> KYSKRIAWMKTTICDSLQLKDMIVEESFQYEKNKNLLEQFLSGEGLNKIFAYYQVQEQAQNDDIKDTGAQDPVLFFTTGDLEKIQDKAVWFLRITNPADDKKKASQQDGNDNDIIFGEITPNTVPMLNALMESVYSRQIDHIITEKIQFWGVAEEEQVLEFQQHSNKFSSEVREAINLMSPGTEHFKLDYEAISGLSESEKMQHYEMKFNEWINLISSQLNDDSEVRKDEKDAGPATELIYWRSRMQKITNWSEQLKSKDFQIVKASLQRHKNHDNQRPRGDESLSKLMMEYNRLDLLLTDKLNEAKDNVKYLTTLEKFIEPLYNGTPQQIIDTLPALMNAIKMIHTIARFYNTTDKMTGLFIKITNQMIKNCKDRILNKKDNGDNPSLYKMIWEQDPAELIEVLGSCIKLYCEYKKCYNDTKEKVADMPKGKTFDFSDAQIFGKFDTFVRRLQKLIEIFSNIQQFNALAKHNLEGMDVLTNKFKKIIDDFKKKGHNLLDTANNKFDRDWVEFNVEISHLDGELQNFIDNNFNRFRNIEYSLKLLHKFQSTIKRDSLKHNLTSRYNAILHNYATELDTIQRVFQDQKSNPPLVRNMPPEAGKIIWARHLFQKITGPINIFPENVINSTEIRRYYGSYNTLGKQLTIYEMWFYQDWVNKIEQSKAALQATLIVRHDENKKLYVNFDLEIMQLIREAKCLDRQGIEIPESARIILLQEDKFKTYYNELLYALKEYERINSKIKPICKNLLLPHIEDLDLKLRPGMVTLTWTSMNIESYLYYVHQGLKKLEQLIINVNDIIENRIENNLKTVSKVVLVHLPQDTKPLSLDSFVQLQEEYINSKTDFLTSKNVEVERAVDDLLQTIMLYPLDPHVDPVLPEETKRIKRYYFWYFYQALLNSTQNSLNAMKYRVCGKKIPGANTLQNLKPFFQVEVQLNGDKVTLNPSLQEIQKSINRAATAVLRCSKHLYNWDQQNKDSTDKATFYDMIACDKEIVKVILLLTGSIQGTKNKVNEFLSGFTKFEWLCKESIQESIKKFSKNGPTLQNYEDQLKKFSQIEEEIEKIVPTYKIGAMELMTHNICTSLSTWAKEWKLQYSQDLHKRARQLLDSLTEQTKMLSTKLSKPVKDIDSLGYVMETLEQIRKEQAEIDMKFNPVQEMYSLLDNYLPGGITDKDEMDARSLLRRNWDILIQQAEIKGKEYQHKQAIYLKELKQSIKDFTNQVSIFRRDYEKNGPMVEGISPAEAMERLRRFEDEYDVKYQMYKINARGENLFGLQNQKYPELEKTDAEIKNLNKLYNLYDSVIKNIQQFKEKSWQDVSKDDLAKMEEDAGKYGEQCSRLPKDLKEWQAYRDLKNYIDSLREQLPLIISLKKPSIMPRHWEKIKEITNTKLNYENPDQFYIEEIMGAKLLDFREDIEDITESADKQLKIRTGLDEINLYWNDMQFQFGIWGKRDVPCMLNGLIVGTILERLEEDQLQLSTFNSQRHVTPFKAEVENLIRTFSDVNDTLDMWVKVQKLWTSLEPVFTGGDIARQMPLQAKQFQGIDKNWMKIMEKAVETKKVIPCCQNDMLKDFLPDLNRKLEDCQKMLEAYLEGKRKKFPRFYFVSNPTLLKILSQGSEPTSIQEDFEKLFDAITKVTFESAKDKKNPALKQITQIQQVIGRNEENISLTGYYVKCEGNIEDWLKKLEQNMQQTLKDIASAAAQQVFQVGLKEFVSSQASQIALLGLQILWTSKVNEGLERLSRNERNAMDIKRNEIKEHMNILSSMCLEDLNGAVERTKVETLVTIQVHQKDISMDLKCKDVNDFEWQKQTRIAWKTDIDECIISITDWDSPYSYEFLGAKERLCITPLTDRCYITLAQAMSMYYGGAPAGPAGTGKTETVKDLGRTLGVFVVVTNCSDQHRYRDMAKIFKGLVQSGLWGCFDEFNRIDLEVLSVVAMQVESITTARKQHMKKFMFPEEEIEIELIPTVSYFITMNPGYAGRQELPENLKVLFRGVSMMVPDREIIIKVKLASVGYLQIDLLAKKFNVLYRLCEEQLSKQRHYDFGLRNILSVLRTAGNTKRQEIKSDEEMLLMRSLRDMNLSKLVADDIPLFNGLLADIFPKLKEVPKKLYPDVEKKIPEEINAESYLINTPSFQLKIIQLYETCLVRHGFMLVGPTGSGKSTIMKILTEVLTKLGSPHKIVIMNPKAITAEQMYGVKSEISDDWIPGVFSTIWAKSNNRALKHTTWITCDGPVDAIWIENLNTVLDDNKILTLANGERIAMTENCKVVFEVENLNNASPATVSRCGQVYVSPTDLGYEAVIEGWIRNRKASGRAEESDKLGNILRKYLINMRFIELQSKECKEPMMDTSPVISVINILNLLTGCLQYFVQTQRTLSEQEYEKFIVYSMAWAIGGIYEAQDRVRFHELLLAKNAPIPQKGKENETVFDYYVSQDYLDWKICSPEEWVPPQSLQFSQLLLPTLDSFRAEMLLNFILTQPKSHTCSNSALLIGGSGTAKTSSVLLYCNKFDPQKMLFKRTNFSSATSPFMFQSTIEAECDFKVGKEFAPPGNKMMTIFIDDMSMPFVNKWGDQITLELVRQLIETGGFYMLDKTQRGNQRKMKNLQYIGAMNHPGGGRNDIPNRLKRQFFIFNMILPLSIEGIYGPIIKHMFKQKYFSDSTYKVIESLTSATIALWNKVKSTMLPTPAKFHYVFNMRELSRIFKGILTCKKDTINDAPKSMKIKPELFLVGLWRHEAERVLADKLVNNKDKDTVMGYIQEVSLESFSQIENEILEKYSSEKTFLFCDFLRPDVINEDGIIEEEAPKIYEAIDSLTELRKRCNFLLSFYNDRNPSKKMPLVLFDDALKHLLRISRIIRQPRSSGLLVGVGGSGKQSLTRLAGFIGKNLIQQIIVTKTYSDKDLKEDIKKGFDDAGHLGKQVTFLMTDSEVKKEEFLEYINMVLSTGEIPNLLAKDEREVWLGDISQ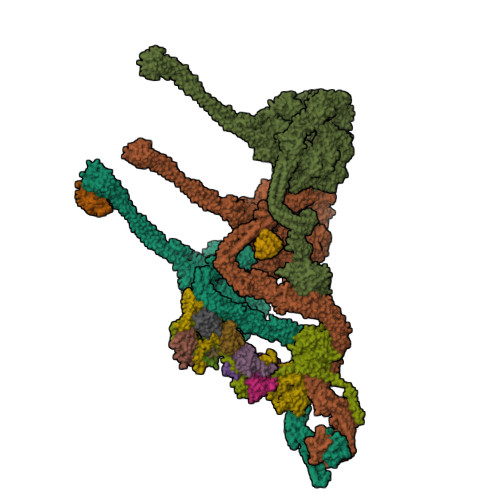AYCKEKNLGNIDPPQSELWTYFVDRVRDNFHIMLCFSPVGQKFRERARKFPALFNECTIDWFLPWPEEALVSVAETFIKNFDKLDTKEETKQELMKHMGNVHLMVNEICDEYYQKMRRQVYVTPKSFLSYLNSYKTLYIEKYDELDQQEESFKIGLNKIQEATITINQMEISLKEEEIQLNEATEKTNQLLANLDKESKKANQKGEEVAATNKQCEIQAEQISKEKEEAERELEAALPALRRAQEAVDSIESKDIVELKANKKPLDIIKYIMDAVLVFFKARLIPIQIEERVFNKKEGKAVLFLKESYDESGIQTLGDMNFMKKLKEFEKDSINEETIELLEPYLNQSEDWFNDTFATKASKAAAGILKWAFAIYEYHQKSKIVKPKRIQVAIAEGRQAIALKELEKAREDLAQIQAYIKNLKDVYTKQMEEKNELEMKAAKTKKKINTARTLITSLSGEKDRWGKGAQDISDQKRKLVGNVSLSTAFISYCGPFNAEYRNKLAQQRFVVDMKKRGVPVTPGLELTSFLIDDATIGEWNLQGLPKDDLSIQNGIMVTNSARYPLFIDPQGQGQNWIRNKLSASIIPERCITTLSHPKFKDMFLKYCMESGLTLIVENIENEVDPMMDPVLERQIIVKGKTQFVNVAGTEMELSKEFKLFMTCRLANPSFSPELSAKTTIIDFTVTQSGLEQQLLGKVISKEQKALEDSLNQLLADVNQNQKDLQRLDKNLLERLINSQGNLLDDTELMDVLNNTKTQAKEVAAKLIDAEIKTKEINEKREQYRPVAIRGSAIYFTMIEVSLVNWMYNSSLEQFLKLFIESIDLSEKAQLPSNRVKNIISFLTFHVYRYVNRGLFEKDKITFILMMAFKILTTAGTISSGDVSLFLKSGDALDIKSERQKQISYLEDNQWLNILALSKHTFSGQTLPFFKELPDLISRSENQWRNWIDKNDPENFPIPDFAESINQEKEIGSFISLCLVRSLRNDRTLIATQNFISNVLGKEFTDPISYPIEGIWQESSNMDPVLFLLSAGADPTSSIDELAKKKKKFPCEKVSMGEGQERVARQVIMKGFVEGGWVILQNCHLGLKFMEEIETLVSPINQIHEDFRLWITCEQHPKFPLGLLQKTLKVTNEPPKGLKAGLYKTFTTIITQEFIDKVDHSNWRSLIFTICFLHSIVIERKKFGPLGWCVPYEYNYSDLEASLLYIEKYLTNLMSTPQPNSHNLPISMNVVRYMICEVQYGGRITDDLDRELFITYGETYLKDGIFGNDYFFYDIMVDGSGQKFKYRIPQNPSAELIKYQEYIAKVPTVDNPEVFGLHSNADLTFRLKESKEMINTVMETRPKDSSVGGGKTREEIVQDKAKDMLKNLPPDYNDVEVRELVSKLGGPNPKTSTERGMTVPLNIFLYQEVTRMQRVIGLVRKTLQDTILAIDGQIIMTPEILEAINAIYDAKVPNSWLYDPSGAEISWLLPNLGSWSTSLSDRNKQLNDWLRSGQRPILFWLTGFFNPQGFLTGMKQEVTRNHKKGDGKGGEAWSLDDVVYSTTVKEREKEKDIEQPPAEGVYIKGLYLEGCKWSKNGLDDSDPKKIFADLPILHVSAINKKKTNEQDRMSNTYLCPVYKYPKRTDKYLIFRVGLPCEGSNNPSHWKLRGVALLCST;> MGDHSQKDSPEDFIINRLSQALGIQKEKIKKSLETQQDDKGEVTNKDEFQGFIQQDNSTNILWVSGQSEKCTFYYGQLPPIDKFKKKGIAVIKLGLHKLTNENVAKDVVVVEITNNLLEHLNSVFNEIMSPVMQNPLNQQGWTDLVAKDLMEKFNNYVAQVYVLLGQIKGKTMLPLPSHKLTSSDTTPDKDKAHVFEGSIITWTKQIKNVLKLEPEQLLKYGNDPGPLAEIEFWQNKRDNLNLIDSQLKSVEVQNILHFLDNNKSTYTTPFTKLQAEVKKARLEANENYRYLFTLKDLFSKLQESQPSDFPTLYELFIPIMHTILLIYNKSKTYNQPPRLVVLIREICNAIISNAQAFVDKDTIFSLIDSKETTEACDKLQVTLDVCSKFKDAYFEYKAKAGGNWKLTSNALFVRLDSFLERCQDILHLTNTIVQFNKLEKIELGGTKGKTLTESIAQIFKEFEEAVQAFTSVSYDIMNIAEKKFDDDFYEFRSKIKELERRLASVITQGFDDYDTIYGRFKLLDNFEGLLTRPIIADELEKKHIVLLEMYKQDLKQVQSIFLEGKQFVDSMHENAPLFLNMPPIAGALTWCKSLRDRIQEPIEKLAQLGQGITEREEYKDVQKLYTSITKSIKDYEDQKILSWEKEVEDSSQDKLKQTLLCKDENDLIKVNFDPSLVRLLKEVKYFLLLRLEVPTTAKDIYTKAETYRTQIVALDMIVDNYNHIKTCLLPVEEPLVKKKIQDMEEEVKPGIEEIRWKSTNIDQFISKSKSIVDQLFETVNKMKDSLQKIHKSLANFNVKIIERKNRPMSPDDYDQFLKAIFSNKLTIVKDNGNQIQKLVKEVLDAVKADKKQNSWKNYNDYVNVIVIEGISTAIQTALLHLNEQINPVFIKRNDISPLFDIRLELGQSGIQFDPEIGESSNQLTVRNTIRNWINDFFNIAGTIQRLDTTMPGDFLQEIRSFFEIKQCLAMITQNLEWIENECNQFRARFDTYSYLWTEDEQISFNRFLDENEPKDEDGKGGDDDEGENTEKQNPLLKGCRAKIPNLDLFDEKITHLKAIQQEISRIKTPEDISWLRINLQPMKTALDARVTRWIRVYTDFLVNQFRTTQKNLLDFIEKTKDGIKKNPADHENLHDKKLLMSVMKVISDVKDVEPRREGIITRMKEMVTKLKKHNVPITEKGTDDPLQQIDNANSNFIEIYGRVFKVKADIIPLQAEETQNIKRDLDIFMKEVESFRKEFMQKLPFDYTESMGYENINNAYDTIMVYYHKLTAIEGRALEYNNLEKLFELQKSNYKQLKDCMNDLKNLKTMWDAIALIHFQYNDWKTKPWRQIKADILLDTNKTLGTQIKNLPKEIRNFKGYNVIVEKVKNMGTVLPLVSALHSEFMEDRHWSQLKQITGTVFDHNSLSFYFEDILALNLYKYENTVNEIVDVAQKEAKIEKKLKNIEQWWSKQVFEFTEYKETKTFASLDNMMEVLDQHSLDLMGMKSQGKYVEFFYDRVEDWREKLGRVDVVVNEWLKVQKNWKILYNIFLLSEDIRMQLPEDTKVFEGVDKEFKDMMSEVSANPSVVEACTIERRDVLVGWSQAIKKCEKALNDYLEQKKKSFPRFYFLSNQSLLTILSNGQNAPKVCEYLGDCFDGLKTLTFEPPANPAETSKVGIGMISKDDEKVPFSSKFICEGAVEHWLLNLEFRMRETLQEILEGAKNTADLWDSGDKPREEWVEGYNAQIALLTTTIVWTEDVGRAFEDLAGGSETAMKECQKLIEVRLENLIKKVRGDLHILERWKIINIITIDVHSRDVVEKFVIQKVSEAESFAWLSQLKFYWENKPDSDMHLRQTLRFPWEKDKNKNKCIIRIVDWFRFYSYEYIGNAIRLVITPLTDRCYITLTQALNLTMGGAPAGPAGTGKTETTKDLGRAIGIPVMVFNCSDQMNKDSMAQIFMGLSQSGAWGCFDEFNRISIEVLSVVSTQVKCVLDALKEKKTKFSFVEEGEIQLQDTVGFFITMNPGYAGRTELPENLKALFRSCAMVVPDLALICENMLMSEGFTMARVLSRKFVSLYMLSRELLSKQKHYDWGLRAVKSVLRQAGKLKRGDPDMPEDPLLMRALRDFNMPKIVTDDKVIFRRLIGDLFPKLDPPTKQNPELKKIVQDTTKKDMGLVAEELFVTKVVQLAEILEVRHCCFVIGPPGSGKTCVWKTLIKSYINSGEDAEYDTLNPKAVTSDELFGAYTKTKEWKNGVIAVIMKNQVKNEEKYKATHMHKWSVLDGDIDPEWIESLNTVMDDNKVLTLVSNDRIFLTPQMRLIFEISNLRNATPATVSRAGVLFINETDIGWMPYMNSWLERSQINILKQQKEMANMPEYPVIDDVAKSVFYRCFQSYFEQNIDVHDKNRVRHICPMVDIAMIQTICTILDALLIQHLPKLKQMKEEDEKQALEAFFIFAGLWAIGGPVGGGQDDSKDMKEFNTVWKGAAKVKFPEQGLCYDYYYDINENKWNTWKVEDYLPNDQPLFSKIYVATIHTTRLRYMIDIHLQRRKPILFIGSAGTGKTAVVRDYLNSTRPEQVSHKTINFSSFTDSLALQKNIESMVEKKNGRNYGSATNKVLICFIDDFNMPYVDKYGTQSPIQLLRLILDYGSIFNREQLEERKFLQDLLFFGCLNQKSGSFTVDLRLQRNFSVFSMYTPSSDVIKTIFGSILNAHLSTIDDKAQKMAFKLVEATYFTFDKILKNTTAFAPSAKRFHYQFNFRELARVCEGICRTTPGQYSGGDQGKLVRLWAHEMKRTFEDRFIANEHVEFFRRYLTEAISKCIGEFPETENPIAEPLIFTGFVAAHQGLDQQYTQCTIPVLKRVLDDKLEEYNEVKAQMNLVLFQQAMEHVSRICRILDMPGNNALLVGVGGSGKQSLCRLSTFINGFEIDQLVVTASFTINDLRNNLQEIYKKIAKPNSIARVFMITDSQIKEEQFLIPINDMLNSGWIFDLFPKEDMDSLVSGVRNEAKGEGVDVNNLTALTSYFLDKIRKNLKVVLCFSPVGDTMRIRSRKFPGIINNTSIDWFHPWPHEALIDVAFRFLEEIEFPTEEIRQSISLNMAKVHSSIDTANEKFLKLERRYNYTTPKSFLELIDFYKKLLTEKRETIQRQIQRYEMGLNILAETQNKVQGLQEELKVKMVEVNKQREETDILIEKVGKESALAEEEQTIANAEEEKTNVAAAEAEKISKEATEALAEALPALRSAEAAVDCLKKPHVTEMKNLGSPPAGVIVTARVVLILFNQGITLNDPDEKVWKKAVTFMNNPQAFIDKVKSFDGENIEPNIIEQSNKIIQDPSKKFNEKDMAGQSYAASKLCAWAVNIVTFNKIFKQVKPLQDAQKQANEILEEKKKELAIVKQRVAELNARVNSLKRQLEEAEARKMIVEQDAARCQSRLSAAENLVNGLAGENKRWTQNVKFLKENIKSMIGDSLLASAFVSYIGAFSAKLRLELWKNTWLPDIIEKGIPITEGIEPLKILTTEAIKSKWKNEGLPADPMSLENAAIITACARWPLIIDPQLQGSTWIRGKQGENLTTISLSQPKWLGALTSSISSGRAVLIEGIQQEIDATLDPLLQRAVKKNGNQLQLEIGGDPIDYDPNFKLFLMTKLINPHFRPEIAAQCTIINFIVTESGLEEQFIAMVVNIEKNELEMAKQDLVKKQNEYAVTLDKLESDLLQSLSEADPATILDNTELIQNLDKTKKTTIEITEQQQKAKVTEAEINIQREHYRVVAAEGSMLYFLVISLSVMDHMYQYSLESFITFFFKAINRTTVRDENRIPTLILNIRQTIYQWISRGLFEKHKLIFLTLIVFRLMQKKIIDVAYEVAEMDFLIKCPARPGVENTLDWLPNISWDQIQGLINLEEFRNFAHQLEKEAPNRFKDWYNELQPEDQKLPLDWKRLDSMPFKKLLVLRCLRPDRMTISLNNFIRAVLPQGDAFVEMDQKLAFSEILESVINEDSESTIPIFFILSPGSDPVKEVEKIAKKKRIEPGKNFFNIALGQGQDEIARRRIEEGNKEGHWVMLQNIHLMPTWLIELEKILDSYSGEAGGGNSEFRLFLSAEPSTGIPIGILDRSIKLTNEPPAGLKANMKRAWTYFSKEEIEDKDPKIKSILFALCFFHSTLIERRRFGPKGWNMSYPFNMGDLRDSYLVMNRYMEQNQGGKVPFNDLIYIFGEIMYGGHIVDDWDRRLCNSYLFNTMHEQLFDELELFPYIEGKGLSFKVPGQNPYEKYIEHIETSLKQETPLAYGLHPNAEIGFRTDQCKTLFNTLLELMPKEQSRDEKSSDIKSSNEMASDLIKQLLEDSELKNKIFNMEEIKNKIDAENKGPYQNVFLQEIEYMNALLSEIVKDLEEIGQGLSGLLTVSENMEMIIESIALSRVPASWQKLAYPSKRGLQSWLANLFQRIEQLNIFRDDPYSIPRVVMISRFFNPQSFLTAIMQVISRAKAYELNKLYIQTEITKRSIEEIEGAAKEGAYVYGFILEGARWDYQLGQLEESKPKEMFSVLPVTYCKAIPLPPEGKEDKSLYQCPVYKTEDRGNTYVFTAQLKTRFPPRKWILAGVAIIMDVEGVSD;> PLVWTQLKQTGTTQPTARSGHTIITVGKTHIMFGGLDNDKNNYKDGKIAPNNQVFTLKLTQNNCEWRQIACQGDVPLPRCYHASCAISADKMLVFGGSYTSNLRFNDTYILKTTSYQWSKPANQISGGEPKNAESKIGAPQPRYGHSATFFEGKVYIFGGHGGINYQRLAFNDLYVLETENFEWTRLEPKGNPPDPRGGHSAAMMANKPQLMIFGGWSFTSQYSNIMIYDIEKDEWVDPEIAHEIPKWNLSGIMAPSIPSWKYFIFGGSVGSFEEGGNRTNSRFVDDSFVLDIDTLSWSSINLEADETSKAVCKPRPRESASIFYDSGESRAIVFGGWANNWLNDLWALNVSTITGPIFSIKPALGPLTGKTKVLIEGDGFKDTQNISVKFSGGKLEKEVNGTFVNEKEISCETPTFDYPRSVEVTVCMNKGDYTITKSAFTYTKADKTIAYGPGLLTENLIGVQTTIVIQARNGSDEFVVTIRNPAKIKKEEEVKEGDKANTKNTIKEDEEEEGEDEEENKKKKEAEKNDLTGSAVMNYISKQLKDIQEFIENTKENIEIRNKNISELINVMINLEKVRVKNDDDVLTLDTVEEMLNFLKKKKDSDIKKCKKLQEEWKNLAKMAQAVKKDIQNPVKTESDKTKENIKKFEEITLKEYANSLKKESFYKTGVSESFKRIGEVKQKVDEFEVQLNQYEDFARIGSKKLMEQIRTDVSSVEKLWVRIEISEKTMDEYKKMKWGSINSMDMEDEIKKLRKALTDLRGIDKRSNAFIGITEELKKWATFLPLLGELKDPSMNSEDGRHWKKLKDLVKKEFDVSQELMLEIIWDLKLFDYKDGIEEITDQAKQELKMEKALKKIIDFWRDIEFELVQHKNTDIHTLKMSEENFETLEDHQLQINNMLLSKYVAYFEKEVEKWKYDLGSVYDVVQLLLEVQKTWSFLENLFEVKRELPNESAQFVGIDKDMKEIMQKGCDIKNCLKFCTIEGMLKRLENIQAQLKVCEKALNEFLDSKRRAFPRFYFVSVNDLLDILSNGNSPAKINRHMSKIFQAIDNLQLKEDSSGGRPTLKMISCVGTEEVDFSSPRLLQGKVESYLKDVIDTMIGTLKSVANSSFKNFQSMTRKEWLKSDPSQITLLVNNIIWSKAVEDCFLKLQSGDINAMKLFLDESIKQLTELIGMVQGDLSKPLRQKIMCLITIDTHSRDVVHRLINEHVRKAEEFQWQSQLKFYWVDNDAKIKIADARFVYNYEYLGNGPRLVITPLTDRIYVTATQALHLKMGCAPAGPAGTGKTETTKDLANALAKACYVFNCSSEMNYESMGNIYKGLASSGCWGCFDEFNRLLPEVLSVCSVQFKAVTDAIKQNVERFIIEGDEISLDPTCGVFITMNPGYLGRAELPEGLKALFRPITVVVPDLELICENMLMAEGFIEAKILAKKFVTLYMLCRDLLSKQLHYDWGLRAIKSVLVVAGGFKRSEPEIAEQALLMRALRDFNIPKIAFQDLYVFHGLLGDLFPGINIKPKKDLDFEKIITDVCIENKLDPDPEFVLKVVQLSELLAIRHCVFVMGPPGAGKSTTWKILAKAQDKTNKKTTLIDIDPKVVSTKDFYGYNLPSKEWKDGLFSKMLRSLAEQPDTNPKWICLDGDLDANWIESMNSVMDDNKILTLANNERIPLKPHMRALFEIRDLRFATPATVSRAGILYISDEVGYQWRSYVKSWIKQEFSQDQEMSKNLDTLFGKYVPDTLDHIKKHCRFLVPVSPISQVISICKSLQTLLKGDVKNLEYLFVYALIWAIGGALAEKDSIDYRKDFSTWWKGAWKTAVKFPSKGTIFDYYVDQSGDSSKFVEWSKRLENKEFDPQVETMGNITVNTIETLATTEFIKSYLMVKHPSLLIGNSGCGKTQLAKGILKEIVQAKPENYAYQLINFNYYTDSTYLQGQIEQTLEKKAGRQYGPPGKVQLIYFIDDLNMPQLDAYDTQTAIALLRQLADYGHFYDVSKLALKDIINTQVLAAMNPSAGSFFVNPRYQRHFWTISIPFPDNESLSLIYITFLNGHLKRFKSTIQEYSNIIVRASLMLHQAVTQNFRKTAINFHYEFNLRHMSNVFQGLLLSDPNKFTEPDKLIKLWIHECERTYGDRLVSTDNLKTYKENIFDIVKKSFSKFNFSRYFGNNPENLIYCNFIAGINSDRFYDQMPNNEMEKHISEALKEYNDNNAFMGLVLFEDAMKHVCRICRIVLPSSGHALLVGVGGSGKQSLSKLASFIMGYTTFSITISATYSMVDLRNDLQQLYFKCGPKEEGILFLFTEGQITNERFLVYINDLLSSGEIAELYTLDEKEAMINQVRAKVKGEGKPDTRENCWNWFIDQVKKNLHMAICFSPVGDMRRRARQFPALVNCTVIDWFQPWPYEALFNVAKSFLEPVDLGDDKVREAVVKFMPFSFTLVNDLGLKLLEQERRYAYTTPKSFLELISLFTNMLAQKRESLERNKERYETGLVKLKETAEQVAIIEVEVKEKQVEAEAKKKEADAFAEVVGREKDKVEKENSKATIEADKCGLIKQNVEAQKSSTQQDLDAAQPLVEQAKSALNSISKKDFQQAKSFASPPAGVPEVFAATIYLLAGYFNEAIEIDKNKKPKDVSWKSSLKLMKSPEEFMEKLLNFKDVVDANQVANVNIVKNQYLNMPSFTPEQMASKSAAAKGICSWVVNIVKYYDVIQDVEPKRKALKEATEQLEEATVKLNEVEEVVRKLNEELNKLKAENDKAIAERNAAISEAERCARRLNLAQRLVTALSSENERWGKSIIQLEDQLKLMVGDVLVASSFVSYSGPFNKKFRNIMINQNFMKFMKEHTIPMSPDPNPIKILTDESTIALWNKQKLPSDSVSIENGTILTNSARYPLMIDPQLQGITWIREKEKANNLKILRLGSKNINRDLELSIENGYSAIIENMNERIDAILMPIIARSFIKRGKNKIIKFAGKDLILHPNFKLFLHTKLSNPHYPPEIQAEAALINFTVTEAGLGDQLLSLVVARERPDLAKMKIELITQQNDFKIKLKDLEDELLYKLANAKGDILDDIELIENLEYSKKLSVEIAEKVAAAKITEAKINETSENYRPAASRGALFYFLLSDLSKVHSFYKYSLESFIVVINRAIDAISENKIYGKTTMMSPRSLKKRVDELIESLTYTAYQTTRRGLFESHKLIVAAMLCLRVLLRSEELNSDEVDHLIIGKVDVNPTPMPDALKSFLNDNIWAACKALETIHQFQGFCQSLETDVLQWKKWYSEEKAETADLPKAFKELSKFHRLLLLRALRPDRLPSALSQFVHDKMGERYIEQPPFNIFETFQETSKTVPIFFVLFPGVDPTPDVERVAATFDVSANNGRFINISMGQGQEDRAKKALFDCAQKGHWIMLQNVHLMQSWLYGLNGLEGFLESVFASPKTHPNFRVFISSEPPNVLLPLMQIIPESILQGSLKIANEAPQYLKANLRRAYNKFDQEFLDKCDKKPTEFKSCLFALCFFHSLMLGRKKFGTQGWSRVYNFNDGDLTICADVLYNYLSKYDQVPWDDLRYIFGEIMYGGHITDDWDRRTNRTYLKVLIRSELLQQNFNLAPQFKSPDPSKFDYEAYRKYIEEKLPIESPQMFGMHPNAEIGYLTQTCDQVFNTILEVQGGSSGGGASKKDDGVMVTLTDFKTRCPHDFNMLLIEEKVKEKTPYIVVCLQECERMNGLLKEIKTSLEDLRLGLTGALNMTDAMESLQQSLSFNKVPDTWEKKAYFSKKPLSSWFADLIERNIQLQEWCKELVTPTSLCISYLFNPMSYLTAIMQFTARAQGLPLDGITIQTNVTAMKGPEDVVNPAENGAYIHGLFLEGAAWEIGGQGQDGYLIEQKPKELHPKMPVINAVAVPLDKKKKNGQYDCPTYVTSARGQTFVFTANLNMESDDSDPNKWILSGTCMLMSDD;> LTAQELNEDMPSKMLEPKNPQAPKNITVYDYYTRKFKTDELVDQMIVHFSMDGDYIWKESNEYKTQEEIRDTKKALIKEAMRKQESEEPGANHDEEAIKQTLRNKFNYNTRECQTINPSIRERGVSTEPPPSDTICGNITQWEIFDAYYAEIMKDHQIENKKKKEVDQDKKQDQSMYSTSFKRCCKIMERMVVQNDQEDKYHDYRYYWSQGDNLEAGKNEGHLLPIWRFSNEKQRKKNVTSICWNPLYPDLFAVSLGSYDFTKQRMGLICLYSLKNTTHPEYAFNCEAGVMCLDFHPKSAALLAVGLYDGTVLVYDIRNKHKKPIYQSTVRNQKHTDPVWQVKWNPDTSKNYNFYSISSDGRVMNWILMKNKLEPEEVILLRLVGKNEEESTLIGLACGLCFDFNKFEPHIFLVGTEEGKIHKCSRAYSGQYQETYNGHLLAVYKVKWNNFHPRTFISASADWTVRIWDSKYTSQIICFDLSMMVVDAVWAPYSSTVFACATMDKVQVYDLNVDKLNKLAEQKIVKQPKLTNLSFNYKDPILLVGDSHGGVTLVKLSPNLCKSGPEIKQTEDKKAMEEFKNVKIEDYEREKMENL;> KEFNNPINFQDTETRYGGIQNQVVNINQYVQRNPNFIDLDNIAELSEHSVNTERVKTGDRGMSHKEGGWPGNVDPNEAQETGRFKKRIEKDTSFPQAVKDLKEGVEKCIYQNNQIDLLEEYFEGETSEHVVENLSSKTLMLFKDEKEICKRSVSEISWHPEGPTKVAVSYAIMRFQQMPEKMPTQAYVWDLLNPNSPEIKLMSPSAVTNISYNQKIPDQIGGGCYNGLLAVWDGRKGENPIMISPVENSHYEPVTHFHWLMSKTGSECVTTSTDGKVMWWDTRKFEAGPVEKLNIIEGLGENEEIIGGTALEYNVEAGPSKFLIGTESGSILTANKKLKKPVEITTRYGLDQGRHLGPVYSINRSNQNPKYFLSVGDWSCKIWVEDLKTPIIRTKYHGSYLSDGCWSPTRSGAFFLVRRDGWMDVWDYYYRQNEIAFSHKVSDSPLTCIKINQTGGAYHNSGKLCAIGDQDGTVTILELCDSLYTMQPKEKDIINEMFEREYRKEKNLETIKKQQELAKRQVQKDMGSQKEKWEKKKLEMIETAEASFHENLAKNPV;> NADDQLKQLSALEGANGYVIFNESGIPLKRHEKSISHEKAVHIAALVSDLWNVSKKVIQRDLKTPENDIEVIRLRTKHSYEYIITQSGDFTMLAIQLCGKAIEEAKKAAA;> MSEVEDTLNRIKTHKTVLGYLIVNSEGGVVRGAFKDEEESKNIANSIPLLTKKARSVVRDLDPTNDLVFLRIQTKLNEIMVAPDDEFSLIVIQTKG;> SHLDKVQPVIKNSDMSVEMQKEVEEVAKKAIDYCNTDKEIATFIKDDFRSRYHGTWHCIVGRNFGSFVTFERSYYIYLYVGQLAILLFKTG;> KAVTDMDINELRKLMIGKAIINSSDMQGDLLQEAQDVIQSGIENNSAPVLNIEAACKYIKENLDKKFGPTWQCIIGEGYAYDVTVQNNTLLFMFYNGNLAVLIFKS;> QQYKTFMGARVLWPPEAADDILEGAIRETQDALKKFEIAREGQKIAEHLKKYMDDHFDPYWHVFFGKNFGCQAVHNKNRFIYFYIEKTAFLMYQT;> HANEQIIDMPENSEMKSMKNDAFSQAKFAVENYKFENKISSHIKKFFDEKYGPNWHCVVGKHFNAYVSYDSKNFIFFYEGQLAILLYRKG;> EPLPPHIIRFNDMAQHLLKKVIRQADVLIKENPQGLEKDIALNLVKFVKSQPEFKIGDGEWQCIIGKNFGCSLTFDANVLAFFDLLPSRKSILLFKSG;> MNHEPEVKATDMEEDMIKRVKEIAINAVKEYKQEKQIAHYIKYEFDKIDGYGWNCIVGRNFGSHIIHQTKKYIFFKINELCLLLWKA;> TDKEYISEEVQKAIDDSVKQVFGIKDDSSQVTITYNKDKVNLWTQQIIDYTIRGLNKLGKHFKYCVTAILQQTNHAGISVQITAYQDTNTDGSLIQCYEINDIYAIVSVFAMAV;> RKREASLITLNYIKNRFYPSKIQKIIKELFEDRLKGVEYDPNNANQLSERLVLELREKIKRGKVPRYKIGVQVVFGEIKGQGLRIASKCLWDVQNDNYASYTYTSEKVYCTGIVFGCYFE;> TTTVTSEDHFMTFYNENNKKLIVVDVYPGWSGPCTAMYPTYNQLMISIDDFEKRIDILLLDQDKLVTYKNDKFHATCQPKFLFISEGKIIDEVLGTNIPVFIEKVNKYIPLS;> AKGTTCQKAIVNWEAANPGKNPSEAEEIKLIFQIPPIEKMDGPVLNTLTKCKKLSLSSNSIDKMISLNMLRNLEILSLSRNVIKKISGLEDIGGTLRQLWLSYNFIEKLDGLNNCSVLQTLYIGNNRIKNWEELDKLKDLPELENVLFYGNPIYEQVKEDPKLIVLKKLPTLKNVDGYIIDDSVLEKVKQIA>MAPLRTKAVEVLQRNSRGAFTVPAHGLYPYQWLWDSAFIALGWTQVDWERAWQELLCLFDYGQGPDGMLPHIVFHEQSRDYFPGPDVWGREARAQPATSGITQPPVVATVVRYLYEKDPDRDRARERARYLFPKLLAFHRWLYHARDPYRTGLVVIVHPWESGMDNSPAWDKPLSRVPVENLPPYERRDVKHVNPEERPRKEDYDRYLSLLYLFRRLEYDPREIYRQSPFKVVDVGFNAILQRANRDLYALAVLLQEDPYEIEEWIVRGEVGLEALWDREAGFYFSWDLVAGEPIAVKTSAGFLPLFAGTPHQGRASLLAQEAERWGEKARYLLPSVDPTSPFFEPGRYWRGPVWINVNWMVAEGFRDYGFAALAARLKADALA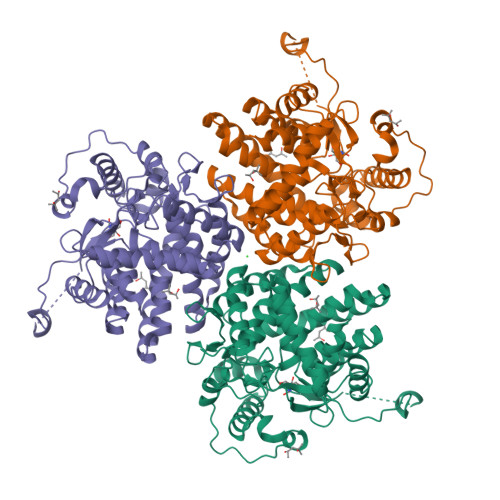LMEREGFREYYDPLTGQGRGGEGFSWSAALALFWTR[2x]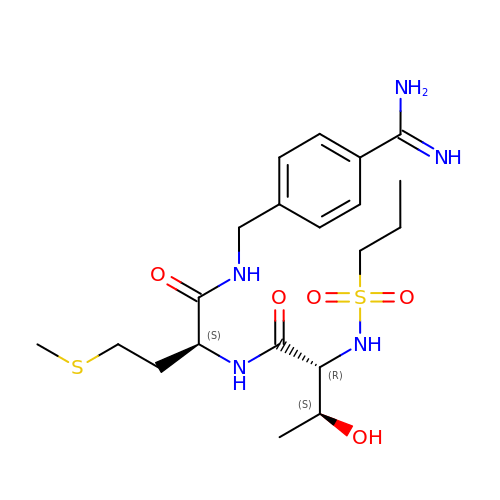N-[DIHYDROXY(PROPYL)-LAMBDA~4~-SULFANYL]THREONYL-N~1~-{4-[AMINO(IMINO)METHYL]BENZYL}METHIONINAMIDE | C20 H33 N5 O5 S2 | AIIJKVORRBMJHS-RRQGHBQHSA-N> TLIELMIVVAIIGILAAIA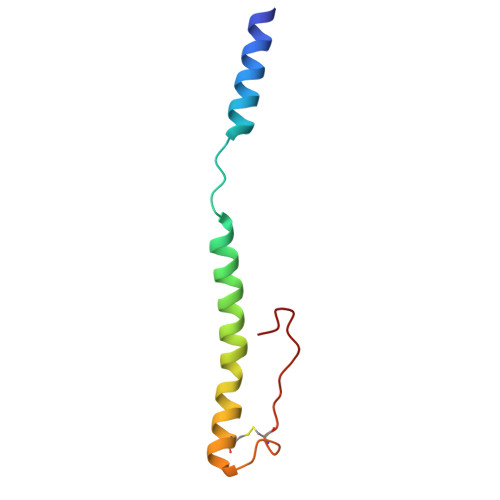IPQYQNYIAKSQVSRVMSETGSLKTVIETCILDGKTAANCELGWTNSNLLG> GAGCAGACTAG;>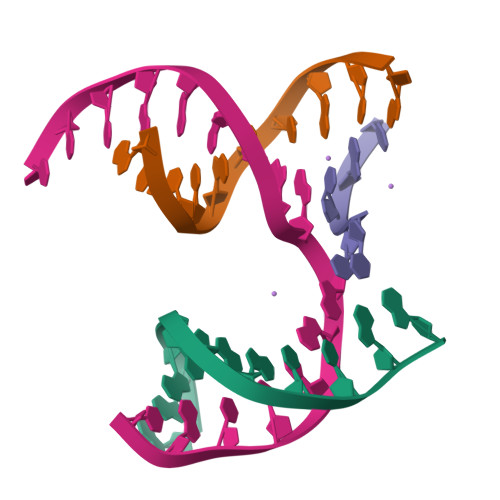 ACACCACTCA;> CTTGT;> TCTGAGTGGAGTCTGC> PDQFRAIIESPEGAGHVGYQYRRNTGSTMRMVSDVLDERVSLWDFHCDPSGNVIQPGPNVDSRQYLQAAIDYVSSNGGGTITIPAGYTWYLGSYGVGGIAGHSGIIQLRSNVNLNIEGRIHLSPFFDLKPFQVFVGFDNGDPASSGNLENCHIYGHGVVDFGGYEFGASSQLRNGVAFGRSYNCSVTGITFQNGDVTWAITLGWNGYGSNCYVRKCRFINLVNSSVNAAHSTVYVNCPYSGVESCYFSMSSSFARNIACSVQLHQHDTFYRGSTVNGYCRGAYVVMHAAEAAGAGSYAYNMQVENNIAVIYGQFVILGSDVTATVSGHLNDVIVSGNIVSIGERAAFSAPFGAFIDIGPDNSGASNVQDIQRVLVTGNSFYAPANITDSAAITLRANLNGCTFIANNFDCRYMVYNAPGTTSPVVQNLVWDKSNVIGGTHANQRAGQNLFDMQFASVVNSTIEV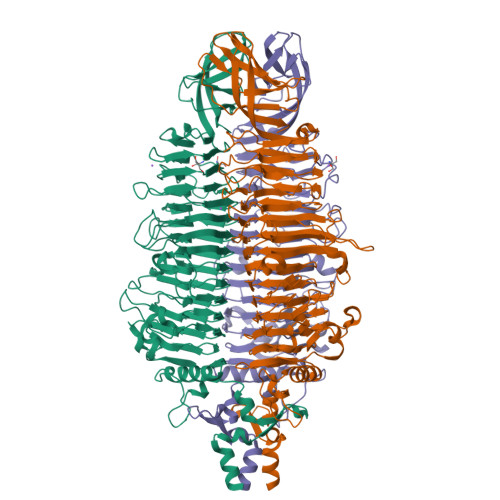QLSCEDLSMFSCILFPASCQLSYSKITVDSAWTKSMSNTAVFEGNQQAGANVYVSYPATVNLTSYNTQGAVPFFSTDTNYAWVTSAYSLSINENLDFSPPATYTNKANGQLVGVGYNEIGGVRSVSVRLMLQRQV> PFGA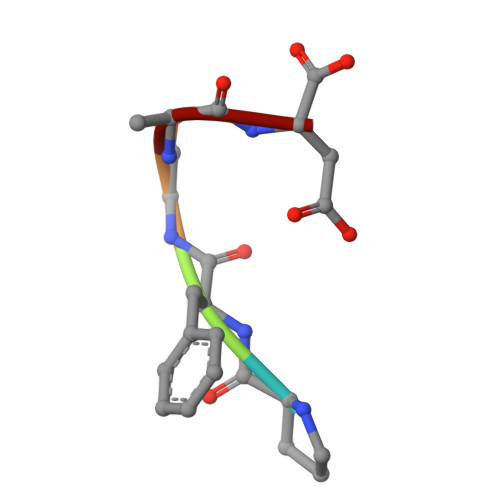D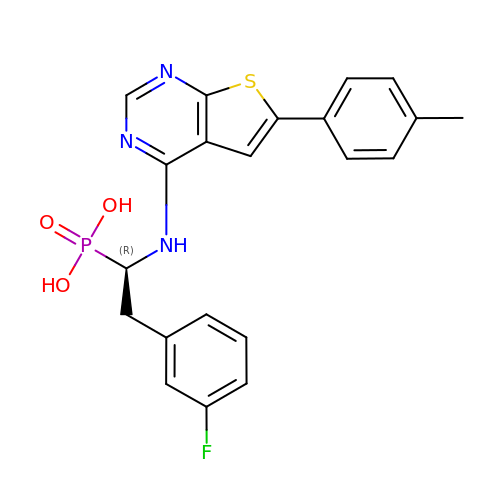[(1R)-2-(3-fluorophenyl)-1-{[6-(4-methylphenyl)thieno[2,3-d]pyrimidin-4-yl]amino}ethyl]phosphonic acid | C21 H19 F N3 O3 P S | ASWGUDOBPNZODI-LJQANCHMSA-N> GPDEEPEEPGRRGSFVEMVDNLRGKSGQGYYVEMTVGSPPQTLNILVDTGSSNFAVGAAPHPFLHRYYQRQLSSTYRDLRKGVYVPYTQGKWEGELGTDLVSIPHGPNVTVRANIAAITESDKFFINGSNWEGILGLAYAEIARPDDSLEPFFDSLVKQTHVPNLFSLQLCGAGFPLNQSEVLASVGGSMIIGGIDHSLYTGSLWYTPIRREWYYEVIIVRVEINGQDLKMDCKEYNYD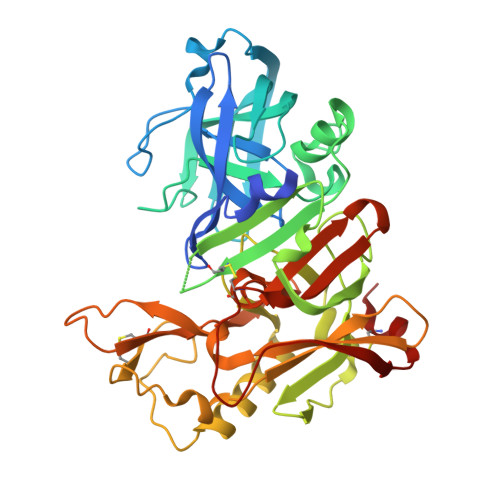KSIVDSGTTNLRLPKKVFEAAVKSIKAASSTEKFPDGFWLGEQLVCWQAGTTPWNIFPVISLYLMGEVTNQSFRITILPQQYLRPVEDVATSQDDCYKFAISQSSTGTVMGAVIMEGFYVVFDRARKRIGFAVSACHVHDEFRTAAVEGPFVTLDMEDCGYNI>[2x]GQS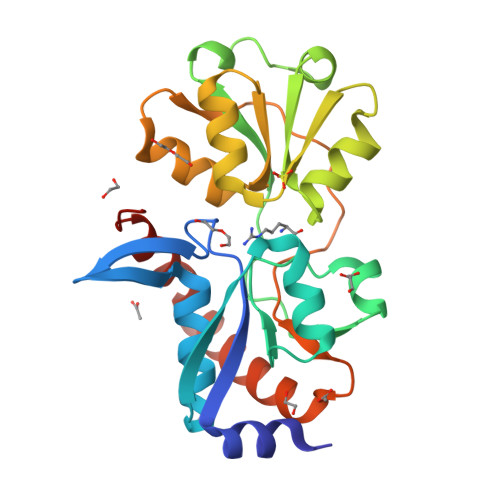AVEAIKQKGKLVVATSPDYAPFEFQSLVDGKNQVVGADIDMAQAIADELGVKLEILSMSFDNVLTSLQTGKADLAVAGISATDERKEVFDFSIPYYENKISFLVHKADVEKYKDLTSLESANIAAQKGTVPESMVKEQLPKAQLTSLTNMGEAVNELQAGKIDAVHMDEPVALSYAAKNAGLAVATVSLKMKDGDANAVALRKNSDDLKEVVDKVIQKLKDEGTYQSYLEKAASLTEVEE4-amino-1-{2-deoxy-5-O-[(R)-hydroxy{[(S)-hydroxy(phosphonooxy)phosphoryl]oxy}phosphoryl]-beta-L-erythro-pentofuranosyl}pyrimidin-2(1H)-one 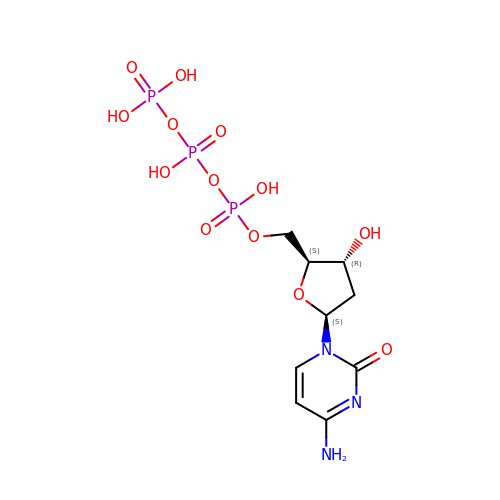| C9 H16 N3 O13 P3 | RGWHQCVHVJXOKC-CHKWXVPMSA-N> EPQVLCYLTSWSSKRPSAGRFMPENVDPTLCTHVIYAFATLKDHKLTEADEKDADMYDKVVALREKNPNLKILLAIGGWAFGSTPFKELTSNVFRMNQFVYEAIEFLRDYQFNGLDVDWLYPRGADDRAAFVSLLKELRLAFEGEAKTSGQPRLLLTAAVPASFEAIAAGYDVPEISKYLDFINVMTYDFHGQWERQVGHNSPLFPLESATSYQKKLTVDYSAREWVRQGAPKEKLMIGMPTYGRSFTLINDTQFDIGAPASGGGQAGRFTNEAGFMSYYEICEFLREDNTTLVWDNEQMVPFAYREDQWVGFDDERSLKTKMAWLKE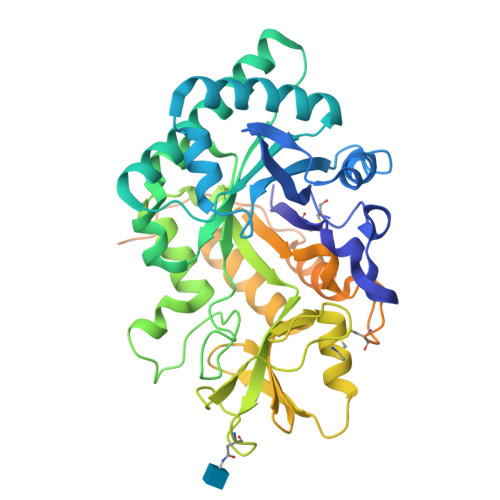EGFGGIMVWSVDMDDFRGSCGTGKYPLITAMKQELSGYKVKLEYDGPYESSSPTGQYTTKDPHEVTCEEEDGHISYHKDHADCTMYYMCEGERKHHMPCPSNLVFNPNENVCDWPENVEGCQQHTQAPAAKR> M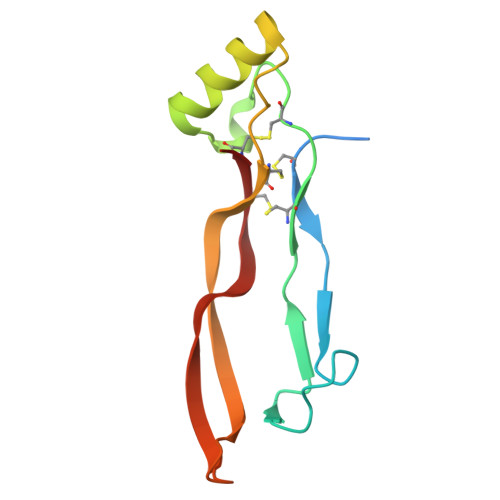AQAKHKQRKRLKSSCKRHPLYVDFSDVGWNDWIVAPPGYHAFYCHGECPFPLADHLNSTNHAIVQTLVNSVNSKIPKACCVPTELSAISMLYLDENEKVVLKNYQDMVVEGCGCR>QKPGETKEVHPQLTTFRCTKRGGCKPATNFIVLDSLSHPIHRAEGLGPGGCGDWGNPPPKDVCPDVESCAKNCIMEGIPDYSQYGVTTNGTSLRLQHILPDGRVPSPRVYLLDKTKRRYEMLHLTGFEFTFDVDATKLPCGMNSALYLSEMHPTGAKSKYNPGGAYYGTGYCDAQCFVTPFINGLGNIEGKGSCCNEMDIWEANSRASHVAPHTCNKKGLYLCEGEECAFEGVCDKNGCGWNNYRVNVTDYYGRGEEFKVNTLKPFTVVTQFLANRRGKLEKIHRFYVQDGKVIESFYTNKEGVPYTNMIDDEFCEATGSRKYMELGATQGMGEALTRGMVLAMSIWWDQGGNMEWLDHGEAGPCAKGEGAPSNIVQVEPFPEVTYTNLRWGEIGSTYQE[2x]

Though often considered synonymous with cellulases, β-1,4-glucanases are enzymes which recognize β-1,4-linked glucan chains which are characteristic of both the cellulosic and hemicellulosic (i.e. mixed-linkage glucans, xyloglucans, and glucomannans) fractions of plant biomass. The catalytic actions of a variety of retaining β-1,4-glucanases contribute to the breakdown of lignocellulosic polysaccharides. Humicola insolens Cel7B (HiCel7B) was chosen as a model β-d-glucanase since it is well-characterized, has good hydrolytic performance with chromogenic substrates, can be readily crystallised, and has been studied in our lab previously. As a tool for the rapid detection and identification of β-1,4-glucanases, a series of glycosylated cyclophellitol inhibitors mimicking β-1,4-glucan oligosaccharides have been synthesised.

Cyclophellitol is an inhibitor of β-d-glucosidases originally isolated from the Phellinus mushroom. This cyclitol is an isostere of a glucoside where the acetal group is replaced by an epoxide. Taking advantage of the catalytic machinery of a retaining glycoside hydrolase, this epoxide undergoes an acid-catalysed ring opening addition to form a non-hydrolysable ester in place of the normal glycosyl-enzyme intermediate, irreversibly inactivating the enzyme. Compound 1 proved to be an efficient covalent inhibitor of HiCel7B, with a ki/KI of 450 M−1 s−1. Intact MS confirmed complete, single labelling after 60 minutes at 25 °C. Binding of the inhibitor had no significant impact on the structure of the active site, inducing no conformational change following addition to the catalytic nucleophile. This is in spite of the epoxide oxygen forming an extremely close (2.3 Å) contact with the general acid/base. Extending beyond the −2 subsite, in which essential hydrophobic stacking with W347 and hydrogen bonding interactions with R108, Y147, and S345 are formed, the active site broadens significantly, suggesting a lack of a specific −3 subsite, possibly accounting for the weak selectivity between 5 and 13.>[28x]A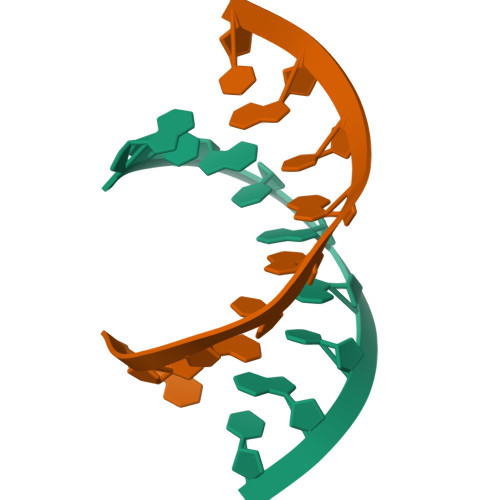UGUGGCAU> MTTTMKISIEFLEPFRMTKWQESTRRNKNNKEFVRGQAFARWHRNKKDNTKGRPYITGTLLRSAVIRSAENLLTLSDGKISEKTCCPGKFDTEDKDRLLQLRQRSTLRWTDKNPCPDNAETYCPFCELLGRSGNDGKKAEKKDWRFRIHFGNLSLPGKPDFDGPKAIGSQRVLNRVDFKSGKAHDFFKAYEVDHTRFPRFEGEITIDNKVSAEARKLLCDSLKFTDRLCGALCV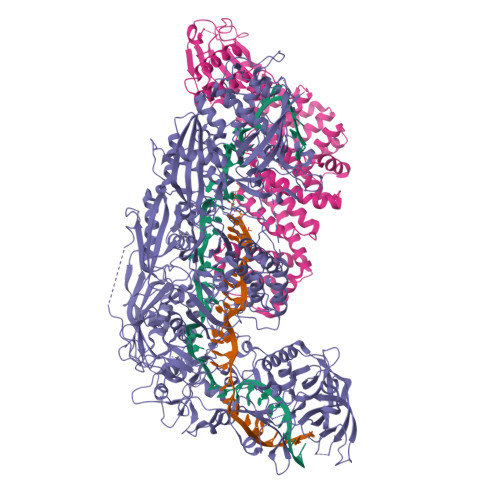IRFDEYTPAADSGKQTENVQAEPNANLAEKTAEQIISILDDNKKTEYTRLLADAIRSLRRSSKLVAGLPKDHDGKDDHYLWDIGKKKKDENSVTIRQILTTSADTKELKNAGKWREFCEKLGEALYLKSKDMSGGLKITRRILGDAEFHGKPDRLEKSRSVSIGSVLKETVVCGELVAKTPFFFGAIDEDAKQTDLQVLLTPDNKYRLPRSAVRGILRRDLQTYFDSPCNAELGGRPCMCKTCRIMRGITVMDARSEYNAPPEIRHRTRINPFTGTVAEGALFNMEVAPEGIVFPFQLRYRGSEDGLPDALKTVLKWWAEGQAFMSGAASTGKGRFRMENAKYETLDLSDENQRNDYLKNWGWRDEKGLEELKKRLNSGLPEPGNYRDPKWHEINVSIEMASPFINGDPIRAAVDKRGTDVVTFVKYKAEGEEAKPVCAYKAESFRGVIRSAVARIHMEDGVPLTELTHSDCECLLCQIFGSEYEAGKIRFEDLVFESDPEPVTFDHVAIDRFTGGAADKKKFDDSPLPGSPARPLMLKGSFWIRRDVLEDEEYCKALGKALADVNNGLYPLGGKSAIGYGQVKSLGIKGDDKRISRLMNPAFDETDVAVPEKPKTDAEVRIEAEKVYYPHYFVEPHKKVEREEKPCGHQKFHEGRLTGKIRCKLITKTPLIVPDTSNDDFFRPADKEARKEKDEYHKSYAFFRLHKQIMIPGSELRGMVSSVYETVTNSCFRIFDETKRLSWRMDADHQNVLQDFLPGRVTADGKHIQKFSETARVPFYDKTQKHFDILDEQEIAGEKPVRMWVKRFIKRLSLVDPAKHPQKKQDNKWKRRKEGIATFIEQKNGSYYFNVVTNNGCTSFHLWHKPDNFDQEKLEGIQNGEKLDCWVRDSRYQKAFQEIPENDPDGWECKEGYLHVVGPSKVEFSDKKGDVINNFQGTLPSVPNDWKTIRTNDFKNRKRKNEPVFCCEDDKGNYYTMAKYCETFFFDLKENEEYEIPEKARIKYKELLRVYNNNPQAVPESVFQSRVARENVEKLKSGDLVYFKHNEKYVEDIVPVRISRTVDDRMIGKRMSADLRPCHGDWVEDGDLSALNAYPEKRLLLRHPKGLCPACRLFGTGSYKGRVRFGFASLENDPEWLIPGKNPGDPFHGGPVMLSLLERPRPTWSIPGSDNKFKVPGRKFYVHHHAWKTIKDGNHPTTGKAIEQSPNNRTVEALAGGNSFSFEIAFENLKEWELGLLIHSLQLEKGLAHKLGMAKSMGFGSVEIDVESVRLRKDWKQWRNGNSEIPNWLGKGFAKLKEWFRDELDFIENLKKLLWFPEGDQAPRVCYPMLRKKDDPNGNSGYEELKDGEFKKEDRQKKLTTPWTPWASSGLVPRGSHHHHHH;> MSNPIRDIQDRLKTAKFDNKDDMMNLASSLYKYEKQLMDSSEATLCQQGLSNRPNSFSQLSQFRDSDIQSKAGGQTGKFWQNEYEACKNFQTHKERRETLEQIIRFLQNGAEEKDADDLLLKTLARAYFHRGLLYRPKGFSVPARKVEAMKKAIAYCEIILDKNEEESEALRIWLYAAMELRRCGEEYPENFAEKLFYLANDGFISELYDIRLFLEYTEREEDNNFLDMILQENQDRERLFELCLYKARACFHLNQLNDVRIYGESAIDNAPGAFADPFWDELVEFIRMLRNKKSELWKEIAIKAWDKCREKEMKVGNNIYLSWYWARQRELYDLAFMAQDGIEKKTRIADSLKSRTTLRIQELNELRKDAHRKQNRRLEDKLDRIIEQENEARDGAYLRRNPPCFTGGKREEIPFARLPQNWIAVHFYLNELESHEGGKGGHALIYDPQKAEKDQWQDKSFDYKELHRKFLEWQENYILNEEGSADFLVTLCREIEKAMPFLFKSEVIPEDRPVLWIPHGFLHRLPLHAAMKSGNNSNIEIFWERHASRYLPAWHLFDPAPYSREESSTLLKNFEEYDFQNLENGEIEVYAPSSPKKVKEAIRENPAILLLLCHGEADMTNPFRSCLKLKNKDMTIFDLLTVEDVRLSGSRILLGACESDMVPPLEFSVDEHLSVSGAFLSHKAGEIVAGLWTVDSEKVDECYSYLVEEKDFLRNLQEWQMAETENFRSENDSSLFYKIAPFRIIGFPAE However, it has also been shown to bind Ter1 sites at the rDNA repeats where it stalls replication fork progression. Here we present the crystal structure of the Sap1 DNA binding domain which allows us to model Sap1 bound to DNA in its proposed replication fork stalling orientation based on structural homology searches and biochemical data. The overall structure of the Sap1 DNA binding domain (DBD) reveals a bundle of four helices, with helices α1-α3 making up a single myb-type helix-turn-helix (HTH) domain. In our crystal structure we have identified a dimerization interface between Sap1 monomers that we predict to be engaged in the direct repeat binding mode.

Since molecular replacement was not an option due to lack of sequence homologs, we attempted to solve the structure by anomalous diffraction using selenomethionine labeling. Unexpectedly however, the structure solution was greatly facilitated by anomalous scattering originating from an arsenic adduct (dimethylarsinoyl) to Cys81, formed due to the cacodylate buffer used in the crystallization solution used in the PACT screen (25% w/v PEG 1500, 0.1 M PCTP pH 7.0 (propionic acid, cacodylate and bis-tris propane)). For comparison we also collected native data from crystals grown in 25% w/v PEG 1500 and 0.1 M SPG buffer pH 7.0 (succinic acid, sodium phosphate monobasic monohydrate, glycine). The two resulting structures were virtually identical, showing that the arsenic adduct did not induce structural changes in Sap1. The packing between the α1, α2 and α3 helix bundle is imperfect and forms a deep cavity. Cys81 is one of the residues lining this cavity and the arsenic adduct previously described occupies the cavity without disturbing the fold of the Sap1 DBD. The structure was solved using a serendipitous arsenic adduct (dimethylarsenate) that bound to residue Cys81. This adduct did not alter the structure and shows that there is a cavity inside the Sap1 protein that can accommodate an organic molecule. The cavity’s connection to the solvent is too narrow in our structure to let pass a water molecule. However, the fact that cacodylic acid, which reacts normally with solvent-accessible cysteines, is found inside the cavity indicates that the pocket may be accessible from the solvent at least temporarily. We speculate that the cavity in Sap1 might play a role in a similar mechanism in S. pombe.

> LSPSSSPAKAQRTHLSLEEKIKLMRLVVRHKHELVDRKTSEFYAKIARIGYEDEGLAIHTESACRNQIISIMRVYEQRLAHRQPGMKTTPEEDELDQLCDEWKARLSELQQYREKF>GAGEGQGPKKQTRLGLEAKKEENLADWYSQVITKSEMIEYHDISGCYILRPWAYAIWEAIKDFFDAEIKKLGVENCYFPMFVSQSALEKEKTHV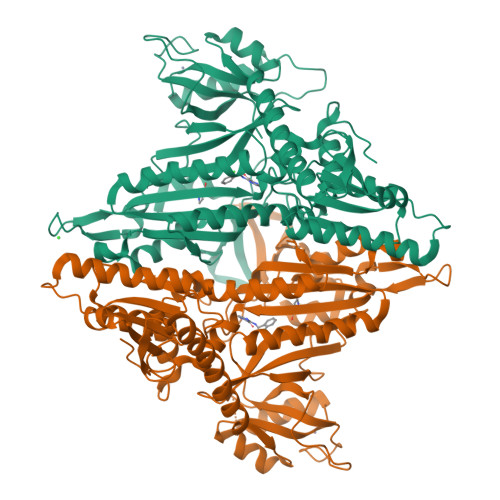ADFAPEVAWVTRSGKTELAEPIAIRPTSETVMYPAYAKWVQSHRDLPIKLNQWCNVVRWEFKHPQPFLRTREFLWQEGHSAFATMEEAAEEVLQILDLYAQVYEELLAIPVVKGRKTEKEKFAGGDYTTTIEAFISASGRAIQGGTSHHLGQNFSKMFEIVFEDPKIPGEKQFAYQNSWGLTTRTIGVMTMVHGDNMGLVLPPRVACVQVVIIPCGITNALSEEDKEALIAKCNDYRRRLLSVNIRVRADLRDNYSPGWKFNHWELKGVPIRLEVGPRDMKSCQFVAVRRDTGEKLTVAENEAETKLQAILEDIQVTLFTRASEDLKTHMVVANTMEDFQKILDSGKIVQIPFCGEIDCEDWIKKTTARDQDLEPGAPSMGAKSLCIPFKPLCELQPGAKCVCGKNPAKYYTLFGRSY[2x]>GGMILLIDNYDSFTWNLYQYFCELGADVLVKRNDALTLADIDALKPQKIVISPGPCTPDEAGISLDVIRHYAGRLPILGVCLGHQAMAQAFGGKVVRAAKVMHGKTSPITHNGEGVFRGLANPLTVTRYHSLVVEPDSLPACFDVTAWSETREIMGIRHRQWDLEGVQFHPESILSEQGHQLLANFLHR[2x];>HMKTLSPAVITLLWRQDAAEFYFSRLSHLPWAMLLHSGYADHPYSRFDIVVAEPICTLTTFGKETVVSESEKRTTTTDDPLQVLQQVLDRADIRPTHNEDLPFQGGALGLFGYDLGRRFESLPEIAEQDIVLPDMAVGIYDWALIVDHQRHTVSLLSHNDVNARRAWLESQQFSPQEDFTLTSDWQSNMTREQYGEKFRQVQEYLHSGDCYQVNLAQRFHATYSGDEWQAFLQLNQANRAPFSAFLRLEQGAILSLSPERFILCDNSEIQTRPIKGTLPRLPDPQEDSKQAVKLANSAKDRAENLMIVDLMRNDIGRVAVAGSVKVPELFVVEPFPAVHHLVSTITAQLPEQLHASDLLRAAFPGGSITGAPKVRAMEIIDELEPQRRNAWCGSIGYLSFCGNMDTSITIRTLTAINGQIFCSAGGGIVADSQEEAEYQETFDKVNRILKQLEK[2x]

Here, we chose aminodeoxychorismate synthase (ADCS) from Escherichia coli, which consists of a class I glutaminase subunit (PabA) and a synthase subunit (PabB), to investigate the mechanism of glutaminase catalysis regulation and its impact on overall GAT activity. PabB catalyzes the amination of chorismate (Cho) to 4-amino-4-deoxy-chorismate, which is a committed step in folic acid biosynthesis. GATs comprise minimally a glutaminase that produces ammonia, which reacts with a synthase-bound substrate to yield specific nitrogen-containing products. As evidenced by analytical gel filtration and isothermal titration calorimetry (ITC) data, the PabA and PabB subunits form a heterodimeric assembly with a dissociation constant KD = 0.16 ± 0.06 μM.

Interestingly, in the ADCS structure without any reaction ligands bound to the glutaminase active site, we observed a metal ion with tetrahedrally coordinated interactions to the two PabA catalytic triad residues aC79 and aH168 as well as to aH128 next to the PabA active site, as evidenced by an anomalous electron density map. As the coordination geometry of this site did not match any of the ions added during ADCS purification or crystallization (Na+, K+, and Mg2+), we searched for alternative metal ions by X-ray fluorescence (XRF) analysis. The resulting data allowed assigning the bound metal ion as Zn2+ that fits well with the predicted coordination geometry. As Zn2+ was not added at any stage during purification and crystallization, the most plausible explanation for its presence is its extraction from the expression host. Comparison of the glutaminase active site geometry in the presence and absence of Zn2+ allowed to identify conformational changes associated with Zn2+ binding. While we did not detect any significant positional changes for the catalytic triad residues aC79, aH168, and aE170, the side chain of aH128 flips from an orientation blocking the PabA active site in the presence of Zn2+ to a conformation, in which it integrates into an interaction network forming the glutaminase active site in a catalytically competent conformation, in the absence of Zn2+. However, our biochemical data did not reveal any effect of Zn2+ on ADCS activity. The associated changes are most visibly illustrated by a long-range movement of residue bE119 from the PabB subunit, which is 10−13 Å from any PabA residues in different ADCS structures devoid of Gln-TE in the glutaminase active site. In all ADCS structures, we found a structurally conserved Trp molecule bound to each PabB synthase subunit, in agreement with previous structural data of closely related synthase subunits or domains of ADCS and anthranilate synthase (AS).>[2x]MRSRRVDVMDVMNRLILAMDLMNRDDALRVTGEVREYIDTVKIGYPLVLSEGMDIIAEF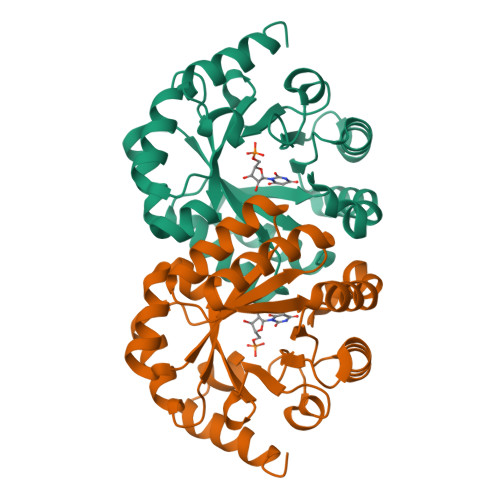RKRFGCRIIADFKVADIPETNEKICRATFKAGADAIIVHGFPGADSVRACLNVAEEMGREVFLLTEMSHPGAEMFIQGAADEIARMGVDLGVKNYVGPSTRPERLSRLREIIGQDSFLISPGVGAQGGDPGETLRFADAAIVGRSIYLADNPAAAAAGIIESIKDLLNP>TTSAVNIYNISAGASVDLAAPVTTGDIVTFFSSALNLSAGAGSPNNTALNLLSENGAYLLHIAFRLQENVIVFNSRQPNAPWLVEQRVSNVANQFIGSGGKAMVTVFDHGDKYQVVINEKTVIQYTKQISGTTSSLSYNSTEGTSIFSTVVEAVTYT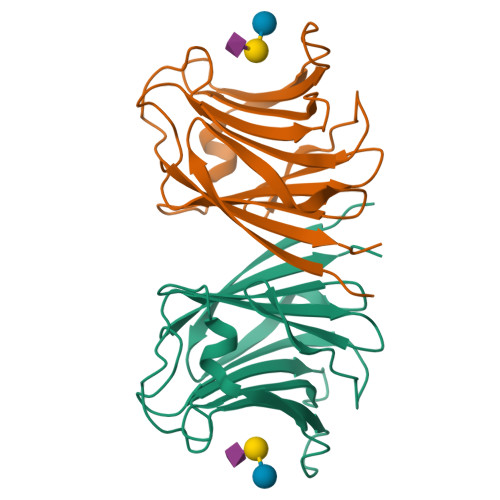GLA[4x]>[3x]MAHHHHHHMLTLVTGGARSGKSRHAEALIADAPQVLYIATSQIFDDEMAARIQHHRDGRPAHWRTAERWQQLDELITPAIAPEEAILLECITTMVTNLLFALGGDSD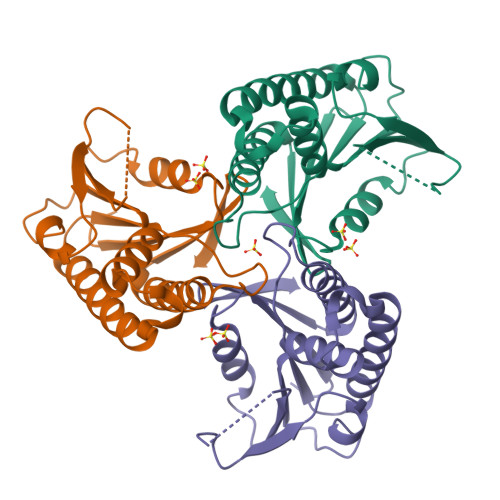PDGWDYAAMERAIDDEIGVLIAACQRCPAHVVLVTNEVGMGIVPENRLARHFRDIAGRVNQRLAAAADAVWLVVSGIGVKIK> SSPSSPLYFEGPSYGIRVSVGSNKQEQQVVLDTGSSDFWVVDSSASCQKGNCKQYGTFDPHSSTSFKSLGSSFSIGYGDKSSSIGTWGQDTIYLGGTSITNQRFADVTSTSVNQGILGVGRVETESANPPYDNVPITLKKQGKIKTNAYSLYLNSPGAATGTIIFGGVDNAKYSGKLIEEPLVSDRYLAVNLKS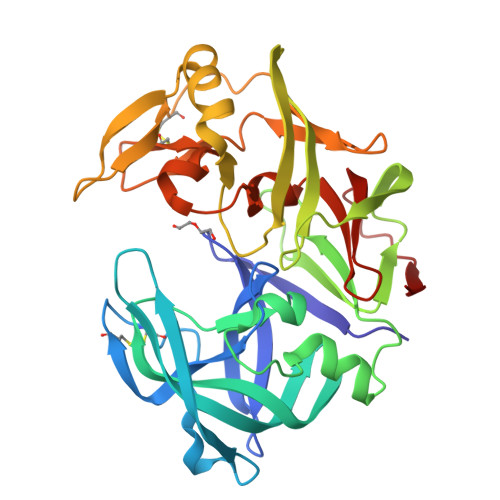LNYNGDNSNAGFGVVVDSGTTISYLPDSIVNDLANKVGAYLEPVGLGNELYFIDCNANPQGSASFTFDNGAKITVPLSEFVLQSTANACVWGLQSSDRQNVPPILGDNFLRHAYVVFNLDKETVSLAQVKYTSASSVSAI> SNAMINVNSTAKDIEGLESYLANGYVEANSFNDPEDDALECLSNLLVKDSRGGLSFCKKILNSNNIDGVFIKGSALNFLLLSEQWSYAFEYLTSNADNITLAELEKALFYFYCAKNETDPYPVPEGLFKKLMKRYEELK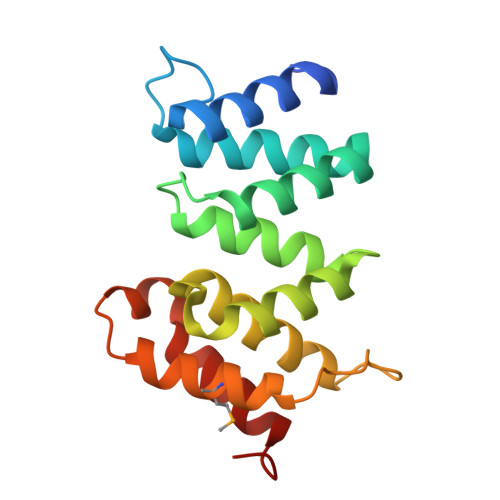NDPDAKFYHLHETYDDFSKAYPLNN> PHMQPFDSGHDDLVHDVVYDFYGRHVATCSSDQHIKVFKLDKDTSNWELSDSWRAHDSSIVAIDWASPEYGRIIASASYDKTVKLWEEDPDQEECSGRRWNKLCTLNDSKGSLYSVKFAPAHLGLKLAC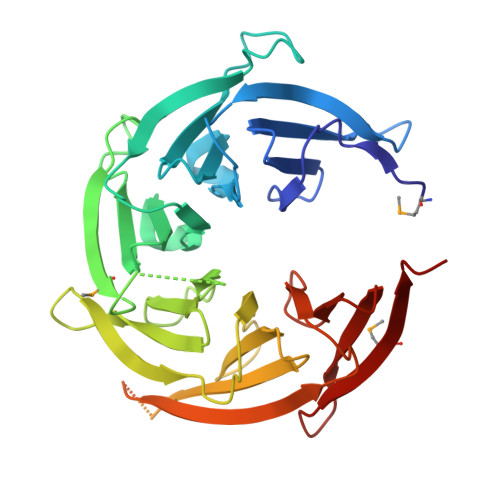LGNDGILRLYDALEPSDLRSWTLTSEMKVLSIPPANHLQSDFCLSWCPSRFSPEKLAVSALEQAIIYQRGKDGKLHVAAKLPGHKSLIRSISWAPSIGRWYQLIATGCKDGRIRIFKITEKLSPLASEESLTNSNMFDNSADVDMDAQGRSDSNTEEKAELQSNLQVELLSEHDDHNGEVWSVSWNLTGTILSSAGDDGKVRLWKATYSNEFKCMSVITAQQ> RKSKAELQSEERKRIDELIESGKEEGMKIDLIDGKGRGVIATKQFSRGDFVVEYHGDLIEITDAKKREALYAQDPSTGCYMYYFQYLSKTYCVD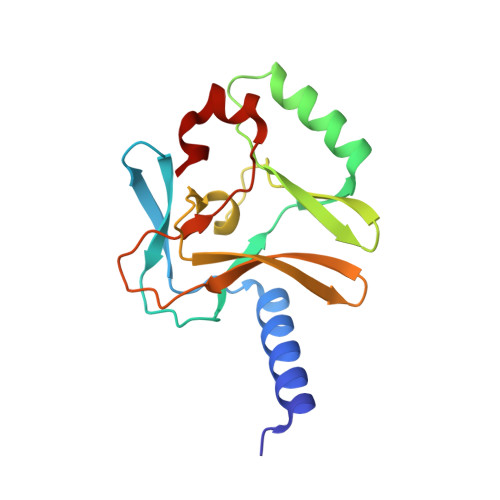ATRETNRLGRLINHSKCGNCQTKLHDIDGVPHLILIASRDIAAGEELLYDYGDRSKASIEAHPWLKH> MSESLTWHDVIGNEKQQAYFQQTLQFVESQRQAGKVIYPPAKDVFNAFRFTEFGDVKVVILGQDPYHGPNQAHGLCFSVLPGVKTPPSLVNIYKELAQDIPGFQIPPHGYLQSWAQQGVLLLNTVLTVEQGMAHSHANTGWETFTDRVIDALNQHRNGLIFLLWGSHAQKKGQMIDRQRHHVLMAPHPSPLSAHRGFLGCRHFS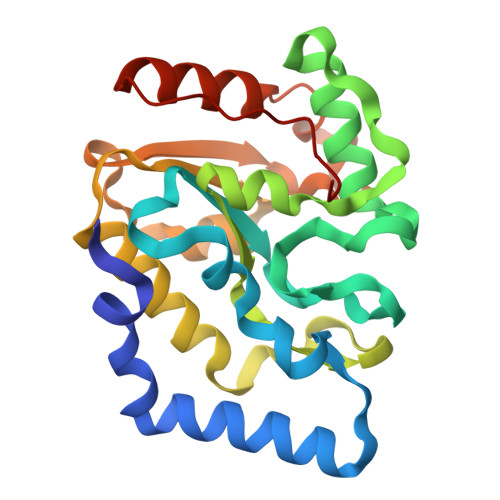KTNQLLQAQGIAPINWQPELES> MDSKHQCVKLNDGHFMPVLGFGTYAPPEVPRSKALEVTKLAIEAGFRHIDSAHLYNNEEQVGLAIRSKIADGSVKREDIFYTSKLWSTFHRPELVRPALENSLKKAQLDYVDLYLIHSPMSLKPGEELSPTDENGKVIFDIVDLCTTWEAMEKCKDAGLAKSIGVSNFNRRQLEMILNKPGLKYKPVCNQVECHPY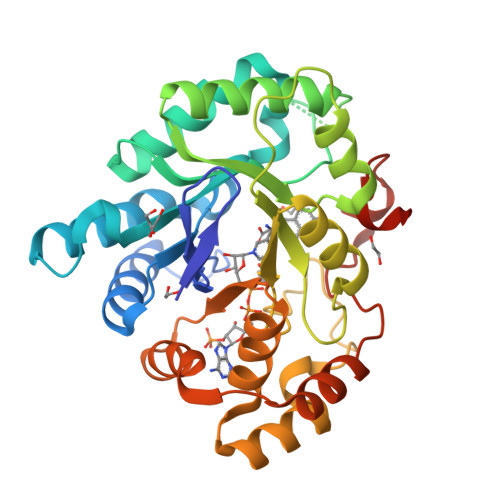FNRSKLLDFCKSKDIVLVAYSALGSQRDKRWVDPNSPVLLEDPVLCALAKKHKRTPALIALRYQLQRGVVVLAKSYNEQRIRQNVQVFEFQLTAEDMKAIDGLDRNLHYFNSDSFASHPNYPYSDEYLEHHHHHH> MARYDKYNPYGGGFRAPLAADWTDADAGKLYAVGINNVGAVVKGAGQSGVAGVLVLTKGAKAG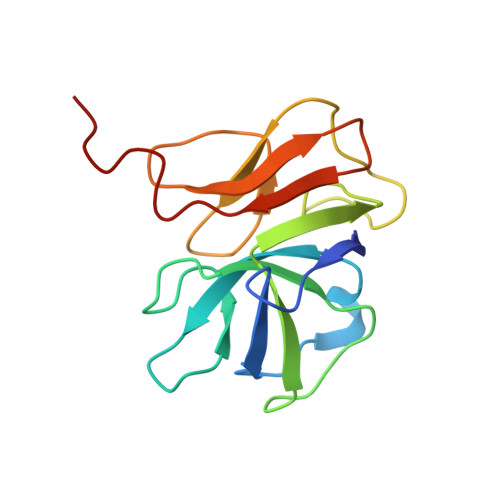SIVDVMKFGEVVEFGPTSGTPGTDFGAAGTAYYADTSTGAINSTSGEAKVKVGHTVGAQRLIVAVADGVVDPSPAA>[4x]MAHHHHHHMNEEYDVVVLGTGLTECVISGLLSVSGKKVLHMDRNPYYGGESASLNLDQMFEKFRGQDAKPPASLGRSRDYNIDLIPKFLMANGKLVKILRMTGVTRYNMEFALVEGSFVYHKGEIHKVPITPTEVAKTPLLGFFEKLKAKKLVSYLYDYDQNNPKTHQGFDCSKDTMDKIYKYYGVSEDTTDF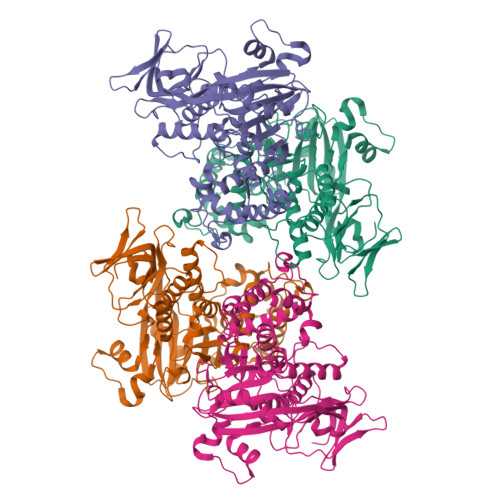LGHAVALYTDDSYMTTVPALEVIERMRLYEDSLNMYGKSPYVYPMYGLGELPQVFARLCAVYGGTYMLDKKVDRIVYDDNGHVVGVESGGEVAKCKMVVGDPSYFPEKVRKTGKVIRVICILSHPVKSTENAKSSQIIFPQKQTGRKHDIYCCVTSFTHHVAPNGKYIAIVSTTVESDNPENEVKVVLDLLNPIDEKFVYILDTYAPLEDGKKDGVFISKSYDATTHFESCAVDIVDIYERITGEKFDWNKKPVEPQEQ>[3x]MNSSIKKIYNHIQEKVINYSDTIDLADGNYVVSRGDGWILSRQNQILGGSVISNGSTGIVGDLRVNDNAIPYYYPTPSFNEEYIKNNIQTVFANFTEANQIPIGFEFSKTAPSNKNLYMYLQYTYIRYEIIKVLQHEIIERAVLYVPSLGYVKSIEFNPGEKINKDFYFLTNDKCILNEQFLYKKILETTKNIPTNNIFNSKVSSTQRVLPYSNGLYVINKGDGYIRTNDKDLIGTLLIEAGSSGSIIQPRLRNTTRPLFTTSNDAKFSQQYTEERLKDAFNVQLFNTSTSLFKFVEEAPSNKNICIKAYNTYEKYELIDYQNGSIVNKAEYYLPSLGYCEVTNAPSPESEVVKTQVAEDGFIQNGPEEEIVVGVIDPSENIQEINTAISDNYTYNIPGIVNNNPFYILFTVNTTGIYKINAQNNLPSLKIYEAIGSGNRNF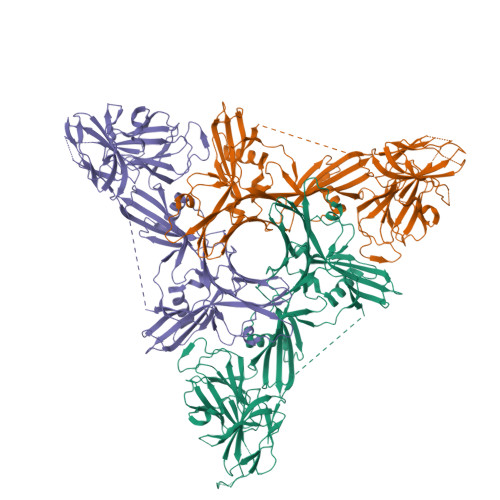QSGNLCDDDIKAINYITGFDSPNAKSYLVVLLNKDKNYYIRVPQTSSNIENQIKFKREEGDLRNLMNSSVNIIDNLNSTGAHYYTRQSPDVHDYISYEFTIPGNFNNKDTSNIRLYTSYNQGIGTLFRVTETIDGYNLINIQQNLNLLNSTKSIRLLNGAIYILKVEVTELNNYNIKLHIDITN> MGSMETPLDLLKLNLDERVYIKLRGARTLVGTLQAFDSHCNIVLSDAVETIYQLNNEELSESERRCEMVFIRG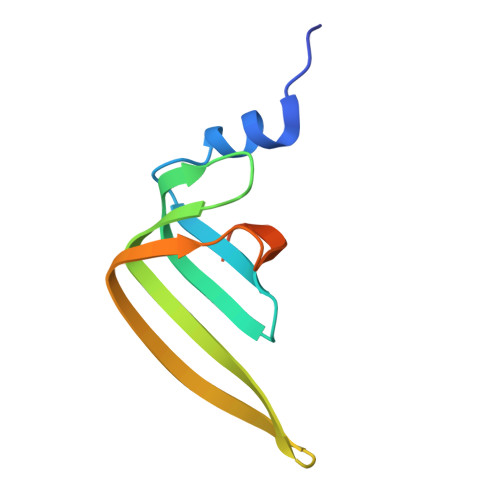DTVTLISTPSEDDDGAVEI(2R)-3-{[(S)-{[(2S,3R,5S,6S)-2,6-DIHYDROXY-3,4,5-TRIS(PHOSPHONOOXY)CYCLOHEXYL]OXY}(HYDROXY)PHOSPHORYL]OXY}-2-(1-HYDROXYBUTOXY)PROPYL 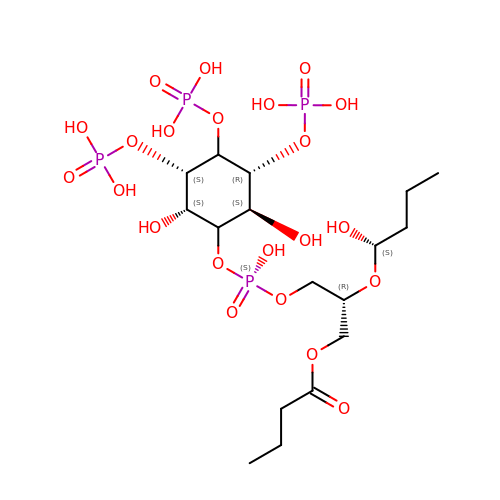BUTYRATE | C17 H36 O22 P4 | JPQZDANYJXWKKH-UASGXTILSA-N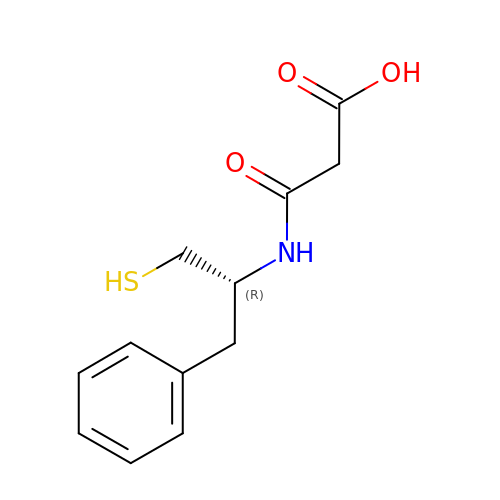(R)-RETRO-THIORPHAN | C12 H15 N O3 S | REPVVNYZORKKPQ-SNVBAGLBSA-N>[4x]MADQAMTDQDQGAVTLYSGTAITDAKKNHPFSVKVGLAQVLRGGAIVEVSSVNQAKLAESAGACSVIVSDPVRSRGGVRRMPDP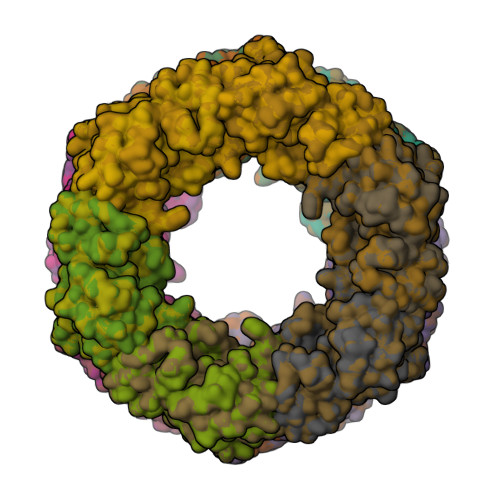VLIKEVKRAVSVPVMARARVGHFVEAQILESLAVDYIDESEIISVADDDHFINKHNFRSPFICGCRDTGEALRRIREGAAMIRIQGDLTATGNIAETVKNVRSLMGEVRVLNNMDDDEVFTFAKKISAPYDLVAQTKQMGRVPVVQFASGGITTPADAALMMQLGCDGVFVGSEVFDGPDPFKKLRSIVQAVQHYNDPHVLAEMSSGLENAMESLNVRGDRIQDFGQGSV;>SPFSVKVGLAQMLRGGVIMDVVNAEQARIAEEAGACAVMALERVPADIRAQGGVARMSDPQMIKEIKQAVTIPVMAKARIGHFVEAQILEAIGIDYIDESEVLTLADEDHHINKHNFRIPFVCGCRNLGEALRRIREGAAMIRTKGEAGTGNIIEAVRHVRSVNGDIRVLRNMDDDEVFTFAKKLAAPYDLVMQTKQLGRLPVVQFAAGGVATPADAALMMQLGCDGVFVGSGIFKSGDPARRARAIVQAVTHYSDPEMLVEVSCGLGEA[4x]>[6x]SHCRLDKSNFQQPYITNRTFMLAKEASLADNNTDVRLIGEKLFHGVSMSERCYLMKQVLNFTLEEVLFPQSDRFQPYMQEVVPFLARLSNRLSTCHIEG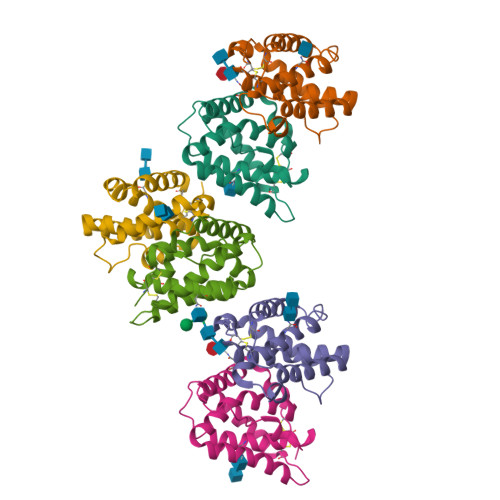DDLHIQRNVQKLKDTVKKLGESGEIKAIGELDLLFMSLRNACI> HHHHHHSSGLVPRGSHMMRSVYPLARRSMAAYTMHNMTVPEPYDYLEDPENP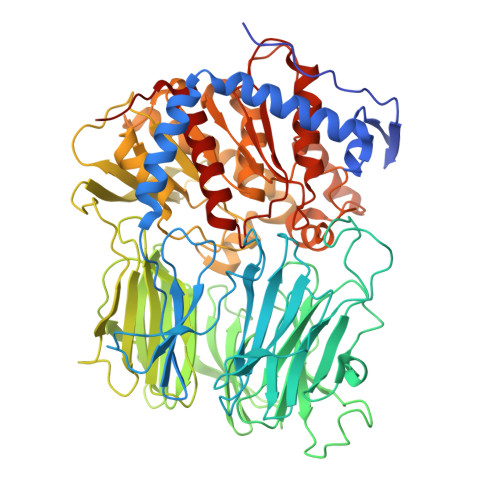ETKTFVNEQNAFFEEYFASEAELRKKIFESISNSQDYPRTSNPSYINGHYYYYHNSGLQNQSVLMRAMSLTDTAPSIFLDPNSMSSDGTTALKATAWSEDESMLAYSLSDKGSDWQRIHVRRADTVEDTSDVIEWAKFTAIAWWHNLGFFYTRYPALQGDVDKGAETDAAQDAFICFHRIGRPQDEDVVILSVPEHPQWNMGASVSDCHSYVIVVLFDGCEPHNLVWVAELPSVEKGLGSEPLVFKKLVNEFAGRYTYLGNEGSTFYFVTTRDAPRKKIVSIDIHTGQETVIVEQQRSVLSQAALVKKTLLLAYLEDVKDVFYYCRLEDPTLNAIPLPIGTITSFFSDRKKDFVSFKITSFLLPGRSFFLDINDPQSSLRVFKDDTVEGLLVDDFVTEQTFYNSSDGVRIPMFIVYRKGSVSSESPLLLYGYGGFNIPLTPAFSSSRMVFLRDLGGVLAVLNIRGGGEYGEEWHDAGRRACKQNCFTDFIEGAKFLHRQGYGSPQTTAIMGGSNGGLLVAAVANQAPELFRCVVCRVGVLDMYKFHKFTIGHAWKSDYGDPEKEEDFRVLQQYSPLHNIKSGIKYPAILVVTGDHDDRVVPLHSLKYVATLQHMNPNEGGPFLARIEVAAGHGAGKPTSKILREAGDIYTFIAKNINASWKE>MTIRSYKNLNLVRANIETESRQFIENKNYSIQSIGPMPGSRAGLRVVFTRPGVNLATVDIFYNGDGSTTIQYLTGANRSLGQELADHLFETINPAEFEQVNMVLQGFVETSVLPVLELSADESHIEFREHSRNAHTVVWKIISTSYQDELTVSLHITTGKLQIQGRPLSCYRVFTFNLAALLDLQGLEKVLIRQEDGKANIVQQEVARTYLQTVMADAYPHLHVTAEKLLVSGLCVKLAAPDLPDYCMLLYPELRTIEGVLKSKMSGLGMPVQQPAGFGTYFDKPAAHYILKPQFAATLRPEQINIISTAYTFFNVERHSLFHMETVVDASRMISDMARLMGKATRAWGIIKDLYIV[2x];>MFEITGINVSGALKAVVMATGFENPLSSVNEIETKL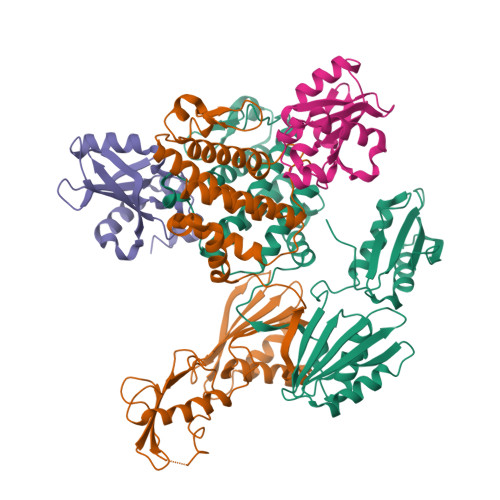SALLGSETTGEILFDLLCANGPEWNRFVTLEMKYGRIMLDTAKIIDEQDVPTHILSKLTFTLRNHPEYLEASVLSPDDVRQVLSMDFAAALEHHHHHH[2x]> MVKFTKQFEGQLVPEWKDAFVDYSQLKKDLKKIHLFTNGVEKKHTETSLIKTVKSSLGRLSIFGNKGREQSRVIQVHKKLASSGSNNDVYETELLEKIADDTDAAKEFFACLDMQLNKVNQFYKTKEKEFLERGECLKKQMDILIELKDAFKQKQANGESTQESKEDDSISCTISCEYDSVRGRTEEMQLQVSCLDNLEDNGEEALESLGSEEPIKANNEDSKLTTVSSRVFSCQGKNVKIKIPLTNPSRTFSAISYLINQSSSKKNGPDGGNKLQISKKKLSHAEKMIKGALTELFKGLNYLKTYRNLNILAFMNILKKFDKVTGKQILPIYLKVVESSYFNISDKVMILSDEVEEWFIKHLAGENRRKAMKYLKPHHRKESHSVTFFIGLFTGCFVALLAGYIIVAHLTGMYRQHSANTFYMETAYPVLSMFGLLFLHLFLYGCNIFMWRKARINYSFIFELGSKNELKYRDVFLICTASMSAIAGVMFVHLSLLEKGYSFRQVQVIPGLLLLGFLLILICPLNIFYKSS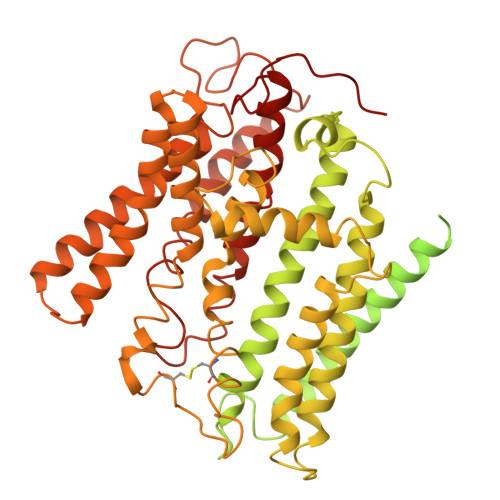RYRLISVIRNIVFSPLYKVVMLDFFMADQLCSQVPMLRNLEYIACYYITGSYATQDYEYCMRVKYYRDLAYAVSFLPYYWRAMQCARRWFDEGETSHLVNLGKYVSAMLAAGTKVAYEKERSLGWLCLVVAMSSVATIYQLYWDFVKDWGLLQHNSNNPWLRNQLMLRQKSIYYFSMVLNLVLRLAWLQTVLHSSFEHVDYRVTGLFLAALEVIRRGQWNFYRLENEHLNNAGKFRAVKTVPLPFREVDEED>TYKKPSDAELKRTLTEEQYQVTQNSATEYAFSHEYDHLFKPGIYVDVVSGEPLFSSADKYDSGCGWPSFTRPIDAKSVTEHDDFSYNMRRTEVRSHAADSHLGHVFPDGPRDKGGLRYCINGASLKFIPLEQMDAAGYGALKSKV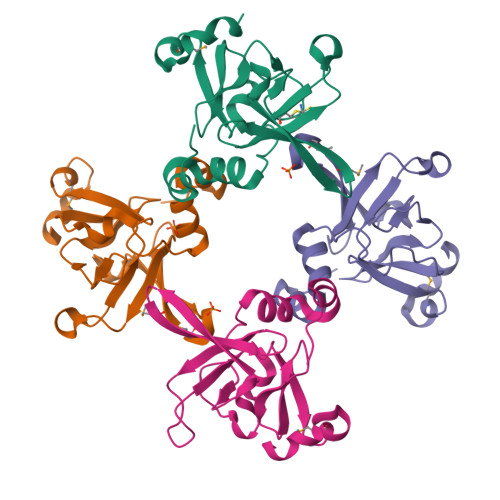K[4x]>ASGSDENDVVIIGGGPGGYVAAIKAAQLGFKTTCIEKRGALGGTCLNVGCIPSKALLHSSHMYHEAKHSFANHGVKVSNVEIDLAAMMGQKDKAVSNLTRGIEGLFKKNKVTYVKGYGKFVSPSEISVDTIEGENTVVKGKHIIIATGSDVKSLPGVTIDEKKIVSSTGALALSEIPKKLVVIGAGYIGLEMGSVWGRIGSEVTVVEFASEIVPTMDAEIRKQFQRSLEKQGMKFKLKTKVVGVDTSGDGVKLTVEPSAGGEQTIIEADVVLVSAGRTPFTSGLNLDKIGVETDKLGRILVNERFSTNVSGVYAIG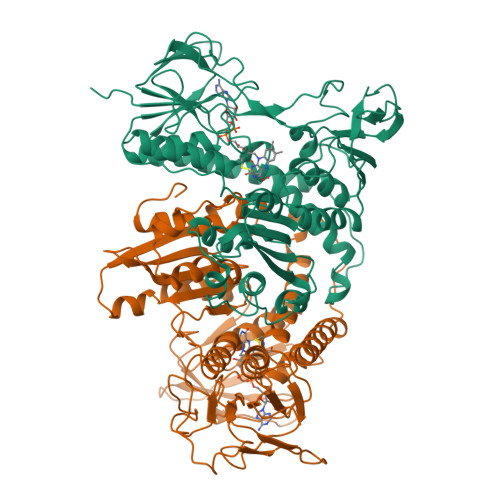DVIPGPMLAHKAEEDGVACVEYLAGKVGHVDYDKVPGVVYTNPEVASVGKTEEQVKETGVEYRVGKFPFMANSRAKAIDNAEGLVKIIAEKETDKILGVHIMAPNAGELIHEAAIALQYDASSEDIARVCHAHPTMSEAIKEAAMATYDKPIHI[4x]>[2x]MQSPPPDPLGDCLRNWEDLQQDFQGIQETHRLYRLKLEELTKLQANCTNSITRQKKRLQELALVLKKCRPSLPSESMEAAQELENQMKERQGLFFDMEAYLPKKNGLYLSLVLGNVNVTLLSKQAKFAY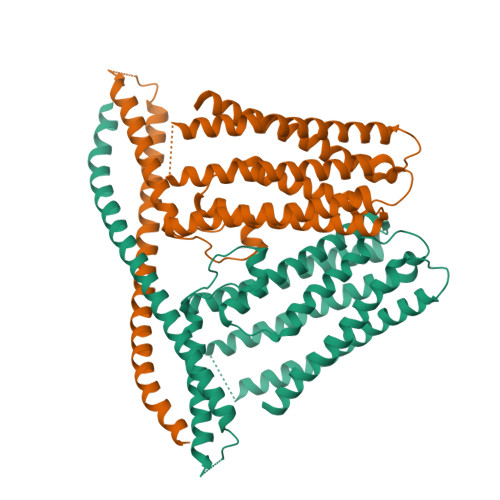KDEYEKFKLYLTIILIVISFTCRFLLNSRVTDAAFNFLLVWYYCTLTIRESILINNGSRIKGWWVFHHYVSTFLSGVMLTWPDGLMYQKFRNQFLSFSMYQSFVQFLQYYYQSGCLYRLRALGERHTMDLTVEGFQSWMWRGLTFLLPFLFFGHFWQLFNALTLFNLARDPECKEWQVLMCGFPFLLLFLGNFFTTLRVVHQKFHSQQHGNKKD>[4x]MIKQRTLKRIVQATGVGLHTGKK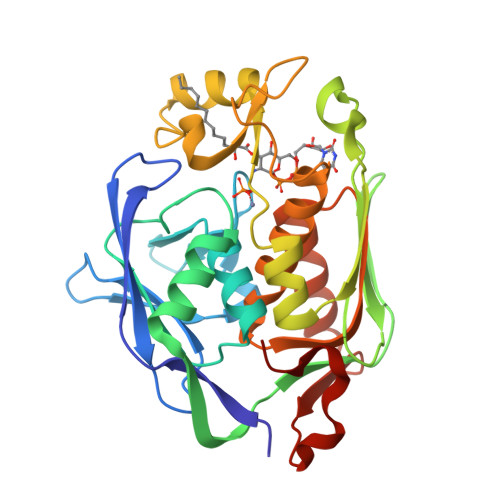VTLTLRPAPANTGVIYRRTDLNPPVDFPADAKSVRDTMLCTCLVNEHDVRISTVEHLNAALAGLGIDNIVIEVNAPEIPIMDGSAAPFVYLLLDAGIDELNSAKKFVRIKETVRVEDGDKWAEFKPYNGFSLDFTIDFNHPAIDSSNQRYAMNFSADAFMRQISRARTFGFMRDIEYLQSRGLCLGGSFDCAIVVDDYRVLNEDGLRFEDEFVRHKMLDAIGDLFMCGHNIIGAFTAYKSGHALNNKLLQAVLAKQEAWEYVTFQDDAELPLAFKAPSAVLA>[3x]LTAKHRPSVVWLHNAECDGCTEAAIRTIKPYIDALILDTISLDYQETIMAAAGEAAEAALHQALEGKDGYYLVVEGGLPTIDGGQWGMVAGHPMIETTKKAAAKAKGIICIGTCSAYGGVQKAKPNPSQAKGVSEALGVKTINIPGCPPNPINFVGAVVHVLTKGIPDLDENGRPKLFYGELVHDNCPRLPHFEASEFAPSFDSEEAKKGFCLYELGCKGPVTYNNCPKVLFNQVNWPVQAGHPCLGCSEP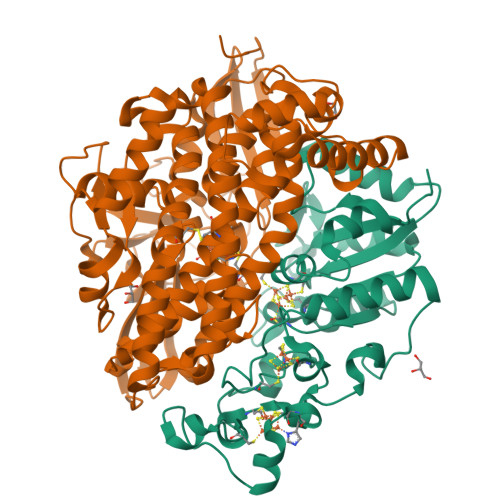DFWDTMTPFYEQG;>ASWSHPQFEKGASGAAESKPTPQSTFTGPIVVDPITRIEGHLRIMVEVENGKVKDAWSSSQLFRGLEIILKGRDPRDAQHFTQRACGVCTYVHALASSRCVDDAVKVSIPANARMMRNLVMASQYLHDHLVHFYHLHALDWVDVTAALKADPNKAAKLAASIAPARPGNSAKALKAVQDKLKAFVESGQLGIFTNAYFLGGHKAYYLPPEVDLIATAHYLEALHMQVKAASAMAILGGKNPHTQFTVVGGCSNYQGLTKDPLANYLALSKEVCQFVNECYIPDLLAVAGFYKDWGGIGGTSNYLAFGEFATDDSSPEKHLATSQFPSGVITGRDLGKVDNVDLGAIYEDVKYSWYAPGGDGKHPYDGVTDPKYTKLDDKDHYSWMKAPRYKGKAMEVGPLARTFIAYAKGQPDFKKVVDMVLGKLSVPATALHSTLGRTAARGIETAIVCANMEKWIKEMADSGAKDNTLCAKWEMPEESKGVGLADAPRGALSHWIRIKGKKIDNFQLVVPSTWNLGPRGAQGDKSPVEEALIGTPIADPKRPVEILRTVHAFDPCIACGVH[3x]>MSTSLKAKVLETFLAKSRPELLEYYIKVILDYNTAHNKVALSECYTVASVAEMPQNYRPHPQRFTYCSQVLGLHCYKKGIHYWEVELQKNNFCGVGICYGSMNRQGPESRLGRNSASWCVEWFNTKISAWHNNVEKTLPSTKATRVGVLLNCDHGFVIFFAVADKVHLMYKFR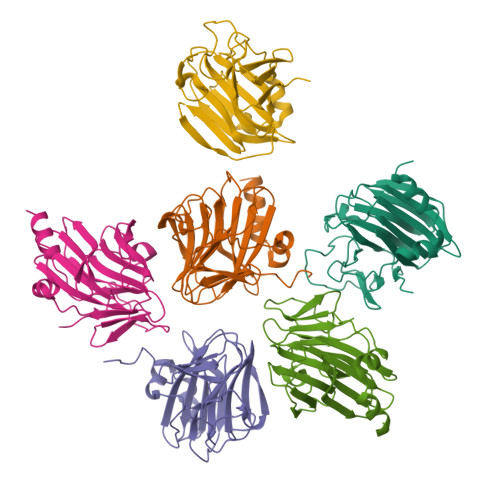VDFTEALYPAFWVFSAGATLSICSPKYLEHHH[12x]1-[(4-aminobutyl)amino]ethane-1,1-diol | C6 H16 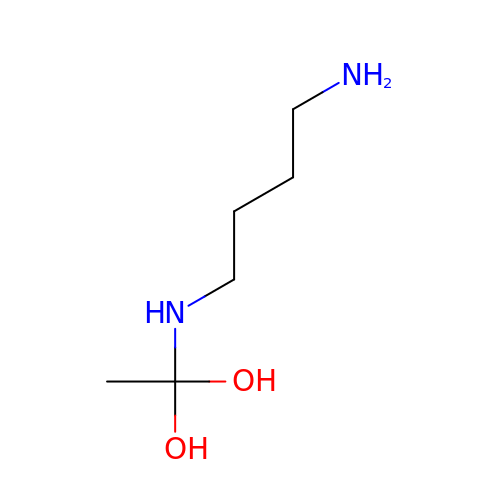N2 O2 | SEXXKOJZDMIAOI-UHFFFAOYSA-N> VDICTAKPRDIPMNPMCIYRSPEKKATEDEGSEQKIPEATNRRVWELSKANSRFATTFYQHLADSKNDNDNIFLSPLSISTAFAMTKLGACNDTLQQLMEVFKFDTISEKTSDQIHFFFAKLNCRLYRKAAKSSKLVSANRLFGDKSLTFNETYQDISELVYGAKLQPLDFKENAEQSRAAINKWVSNKTEGRITDVIPSEAINELTVLVLVNTILFKGLWKSKFSPENTRKELFYKADGESCSASMMYQEGKFRYRRVAEGTQVLELPFKGDDITMVLILPKPEKSL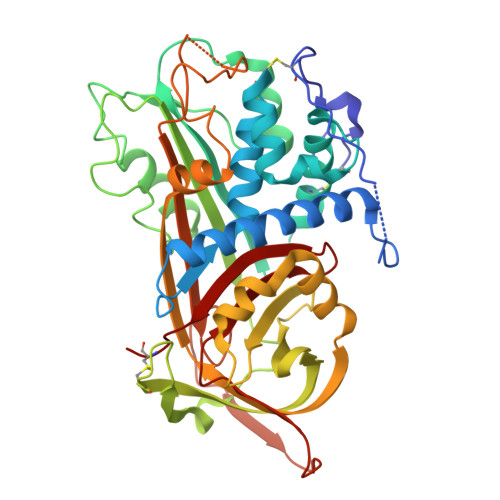AKVEKELTPEVLQEWLDELEEMMLVVHMPRFRIEDGFSLKEQLQDMGLVDLFSPEKSKLPGIVAEGRDDLYVSDAFHKAFLEVNEEGSEAAASTAVVIAGRSLNPNRVTFKANRPFLVFIREVPLNTIIFMGRVANPCV>QANTSYTDYNVEANPDLFPLCLQHLNASFPDCASGPLSLTPVCDRSLSPKDRATALVSLFTFDELVNNTGNTGLGVSRLGLPNYQVWGEALHGVGRANFVESGNFSWATSFPMPITMMAALNKTLIHQIGTIVSTQLRAFSNAGLGGVDVYSPNINTFRHPVWGRGQETPGEDAFLTSVYGYEYITALQGGVDPETLKIIATAKHYAGYDIESWNNHSRLGNDMQITQQELSEYYTPPFIVASRDAKVRSVMCSYNAVNGVPSCANKFFLQTLLRDTFEFSEDGYVSGDCGAVYNVWNPHGYASNEAAASADSILAGTDIDCGTSYQWHSEDAFEDSLVSRSDIERGVIRLYSNLVQAGYFDGEDAPYRDITWDDVLSTDAWNIAYEAAVEGIVLLKNDETLPLSKDIKSVAVIGPWANVTEELQGNYFGPAPYLISPLTGFRDSGLDVHYALGTNLTSHSTSGFEEALTAAKQADAIIFAGGIDNTIEAEAMDRENITWPGNQLDLISKLSELGKPLVVLQMGGGQVDSSSLKDNDNVNALIWGGYPGQSGGHALADIITGKRAPAGRLVTTQYPAEYAEVFPAIDMNLRPNETSGNPGQTYMWYTGTPVYEFGHGLFYTTFEESTETTDAGSFNIQTVLTTPHSGYEHAQQKT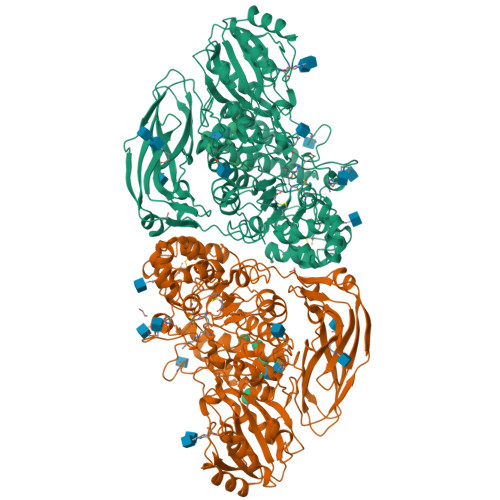LLNFTATVKNTGERESDYTALVYVNTTAGPAPYPKKWVVGFDRLGGLEPGDSQTLTVPVTVESVARTDEQGNRVLYPGSYELALNNERSVVVKFELKGEEAVILSWPEDTTSDFVSSIDGGLDRKQDVIA[2x]> FSTPVDIDIVLADADKRAMVDVKLDKNRREKVPLYMDG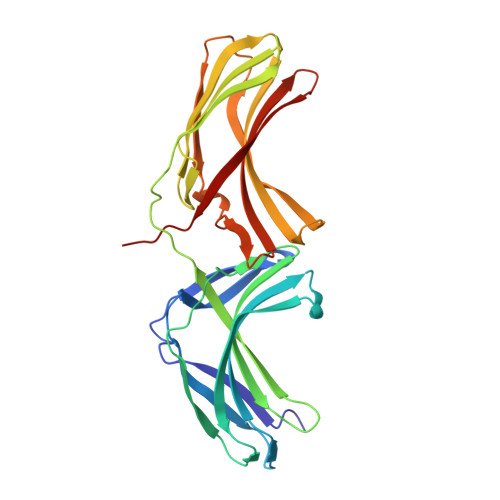ESVKGCVTVRPKDGKRLEHTGIKVQFIGTIEMFFDRGNHYEFLSLVQELAAPGELQHPQTFDFNFKNVEKQYESYNGINVKLRYFVRVTVSRRMADVIREKDIWVYSYRIPPELNSSIKMDVGIEDCLHIEFEYSKSKYHLKDVIVGRIYFLLVRLKIKHMELSIIRRETTGVAPNQYNESETLVRFEIMDGSPSRGETIPIRLFLGGFDLTPTFRDVNKKFSTRYYLSLVLIDEDARRYFKQSEIILYRQPPE>ISLGELGLLPSTVLAIGYYENFVSTVCDALHSLPTIKLNGIEYKDFVFNIIIPND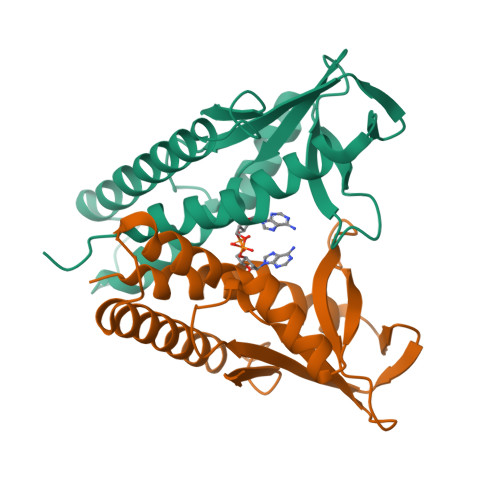LDADIKRRAQIYFKKMDIHEVKIDTNGRSFPLYLQIDEENSGDVAVLYDMPTTLGGIDKAIEMYMKKGHIGKTSQQQLLEERELRNFKTTLINLINNNSFTKTFVKVIEE[4x]Yeast Ddi1 has three structural domains. It has an N-terminal UBL domain that shares only 14% sequence identity with ubiquitin. Yeast Ddi1 also bears a C-terminal UBA domain that is found only in plants, fungi, and invertebrates, but not in vertebrate Ddi1 orthologs345.

We obtained a new crystal structure of the RVP domain of Ddi1 (residues 185–325) at 1.8 Å resolution. The asymmetric unit consists of two chains, which form a dimer with non-crystallographic C2 symmetry. In the new structure, electron density is visible for the N-terminal segment spanning residues 185–199. Intriguingly, this N-terminal segment binds into the active site (Asp220) of an adjacent protease dimer in a different asymmetric unit. Nonetheless, while the observed arrangement is a likely an artefact of crystallization, the N-terminal segment acts as pseudo-substrate and reveals how Ddi1 might engage a substrate. The N-terminus adopts a β-strand conformation that interacts extensively with a loop formed by residues 245–258. There are multiple hydrogen bonds between the backbone atoms of the pseudo-substrate and the loop, suggesting that it might be involved in positioning the substrate for catalysis. The side chain of Phe246, which is conserved as an aromatic residue across Ddi1 orthologs, interacts with a methionine in the N-terminal fragment, suggesting this may be a specificity determinant for the protease activity of Ddi1. In Ddi1, the flap does not wrap around the pseudo-substrate, thus leaving it solvent-exposed. The structure also reveals how Ddi1 could cleave a peptide bond: the catalytic residue Asp220 holds an ordered water molecule in place, which may act as the nucleophile for peptide bond hydrolysis.

>[2x]GPLGSEQLRNAIEYTPEMFTQVPMLYINIEINNYPVKAFVDTGAQTTIMSTRLAKKTGLSRMIDKRFIGEARGVGTGKIIGRIHQAQVKIETQYIPCSFTVLDTDIDVLIGLDMLKRHLACVDLKENVLRIAEVETSFLSEAEIPK5'-deoxy-5'-piperidin-1-ylthymidine | C15 H23 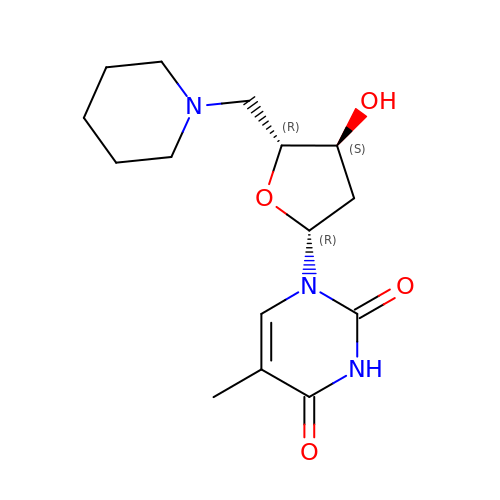N3 O4 | GMOUOGHZJCSNOZ-YNEHKIRRSA-N>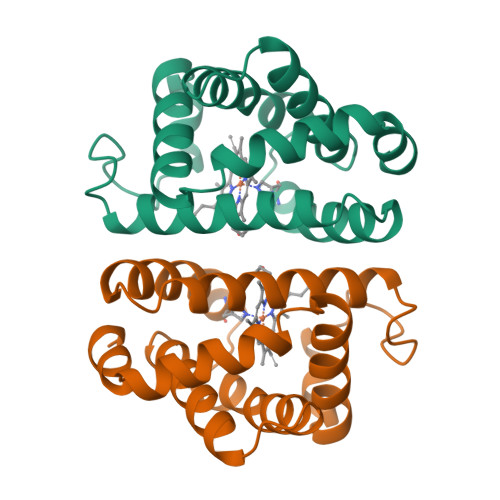[2x]PSVYDAAAQLTADVKKDLRDSWKVIGSDKKGNGVALMTTLFADNQETIGYFKRLGDVSQGMANDKLRGHSIVLMYALQNFIDQLDNPDDLVCVVEKFAVNHITRKISAAEFGKINGPIKKVLASKNFGDKYANAWAKLVAVVQAAL> MSTTEQPLNPNKVSAPVEDPIDPLAVDAASTVKAQAQTQITAQEQNDLNRASTTLQNLQKAEDPNADSGIAASEPTAPAKTTTASKTATSAPAVSWTLDGLNNAEWYENIGKGQLPVYARAHVMLNNAHASPGAIDGMSGKNTLKAIASFQQMNGLSPTGELTKETWDALVAKQNKPAFIEYTITDADLKGPYAQSIPSDYALQAKMKGLYYTRVSEMLGEKFHIDEAFLKKINPTATFKKVGEKIIVPNVRNDLPEDIHLIIAHKGAKQLYLFNSRNQMIASFPATIGSTDTPSPTGTYKVVGVARNPWYS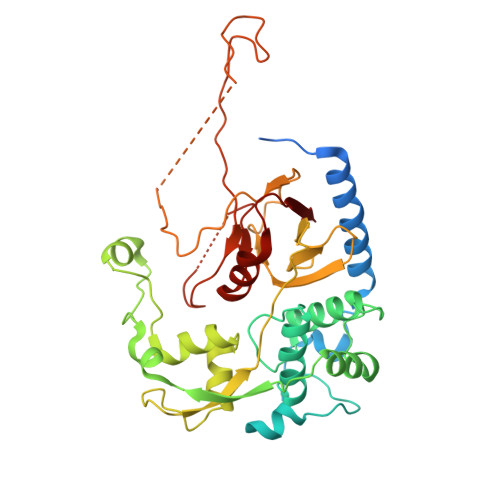YSPSNFVQGKNLKPLSLPPGPNAPVGNIWIGLSKKSFGIHGTPNPSLISKTASHGCIRLTNWDANDLGNKVRSGVTVKFLE> MCKAIYNPEKGLLKHSDLQLEDDKYSDLQLVDEKHTIKRSVESIKSALSLVDDGDLTLSAYDTAWVALIEDVNGRSGFPQFPSCLQWIVSQQLPDGSWGEPLMFLAFDRLLNTLASVVALTKWNIRPDICQKGMKYVLENLNKLVDEKEEHMTPGFELLFPKLIELAQKLDIKMPMDSPALKELYARRDTKLAKIPKKIFHKMPTILLYSLEGMNDLEWDKLLKLKSENGSFLCSPAATAFAFMETKDQDCLAYLTDLVAKFNGGVPTFYPTDMYEQIWIVDRLQRLGIAHYFSSEINNFVDHIYRYWDQKGISFARKCNLPDIDDTAMGFRVLRTHGYQVSSDVFQHFEKDGQFYCYWGQTAEAVTVMFNLYRASQVLFPGEKILDNAKKFAHNFLTEKVATNQVFDKWIITKDILGEVQYALDVPWYASLPRLEARYYLDQYAGDGDVWIAKTLYRLKYVSNNEYLETAKLDYNHCQKIHKLEWSYIQKWFLDLKIEESINTRTLWSYYQAAASIFHPERYNERLAWAKTNVLVDTITTFFSKQQMSKDDIQGFVNQLTNTE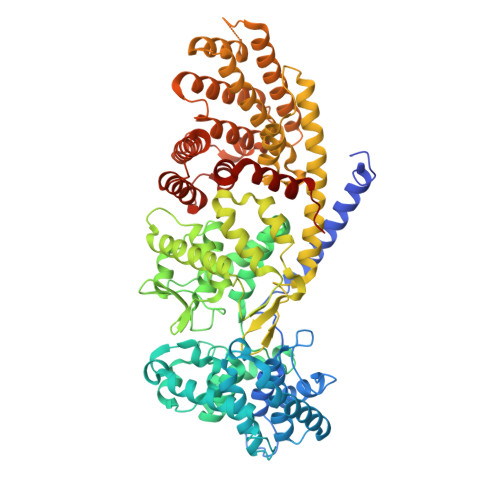NQQTYGKMSHMLIDALNETLKHISMKARETHGIDIYPHLQSSWKKWLLSCMNGPNVAGVAELIVETINLTSGRSFSNDLLSHPQYKQITSITNDLCHQLCSKGNRAIGSEIESKMQELVQLVFSDSSDGLDPDVKKTYLVVAKSFYYMAYFDAKTIDSHINKVLFEMVV> MTPARDLIEKLRLLLNDKDKKSFTDEELNLF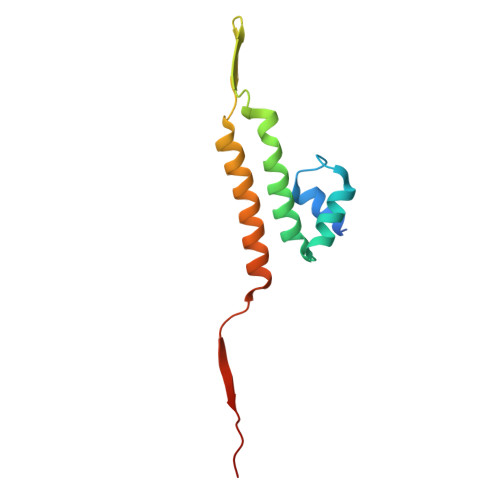LEEADCIYCAASQGWILKSLQYENTVGEMYEYKVGQETYKSSSIKDLVSVAYQNADKFKDMCTNKKEKGSFMLGISTEFEI>[2x]MVKYPKQLFLESKNSKMNSIEMKYGQDPAINRAEFHVYGGVRQSKRKSEAWEAAKRITKERGIPNYNPDLHLKGAQMGQKVLQTYRITGLDREWAGGEDTPAHKGWKPGTDIAGLEMDDLNYENNPAMQQCYDDMRRTAINGLSIAHETIERRFGKEVTPETINLYFEMLNHNIGAGAIMMEHTAETNPELV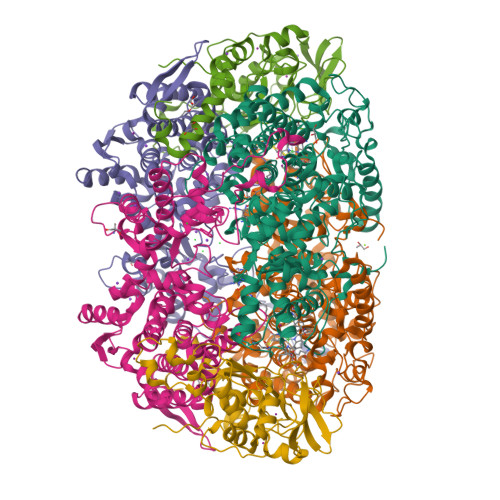KDSYAKCFTGNDELADALDQRFLIDINKMFPKYQADQIKAEVGDRIFQVARIPTMAVRTSDGGLSRAWVGQQASLAFLCAYDIPAGDAVTSDFVFTIKHGDVVFMGTQLPYRRAQRNNSAGGIALGYYSDCNQTSRTPEALEGLDGGIDPVKVIVEALTPGCVITDQGWLHNYLAGGSSGWSNYIISVYTDEVLEDYGYHGAIYAMDKWKCGVGEVPNTYENMMTIAEEVSRWSQKNYDEYPGLMEAHFGGSQRYSIQAAASGAAVGAMTGDPDLGNAAWHYNTPLCKEHYLRLGFYGHDLQDQQNMGHTYSYRSDQGIPYELKGPNYPDFAMNVGHMGGYIGIIAGAAHARGAAYSTNPIIKAAFADPNLQFDFRYPRREFGIGGLRQFMPAGERDAVIPPH;>MAYLTEKIDLYGDNGKVLESDIPLEAVTPVQNPAVRELASIFKRSVAVNLGGAQKALSTGHYANEYIHFPDIPNKDKLGIKSSPGGKYPPKSVKVRTMDLPLVDDADDIAARLKERLQVNPDDGTEVRVMKKGNVLYVKISEQLANTGVEYTTALTTTAQAMTDLVMEKYDLDFHASPLVHCAFYGRYPQTYEFMGGNVISLLAASCANEGPGFAMRNIMANHIVAATRKRTLEAVALSSTLEAIGHVEMGDAIGRWRRWQALVHACQGLNANNVVYDLVKEAGHGCTGDVVAATVGRALEDGIISVKKTLPSGYKFYTANDPSMWNAYVCAGLVAAVIVNQGAARAAQGVSSTLLYFNDLIEHETGLPHAGYGDGMGNGVSFSFFSHAIYGGGSPGIFSGNHIVTRHSKGFAIPVIAAAVSLDSGTAVYGPEATSGLVGDIFGEVDLIRRPMEAIASAAAEIKDKF[2x];>[2x]MVYQRQFLPADDRVTKNRKKVVDPSVKLEKIRTLSDKDFLTLIGHRHLGEAYRSVNPPLAEIGEPEDPIRELVPPTEGAKAGDRVCTIIMTDSVYNPPIAHYTRAWMYHNRFRGIDNGVYSGRVTLEMRERDLEEACRTLFETEICDASRDQVRQYTCTGHSCRLDPDGMMFDPIERCIMSGGNVVYQKDSFGNPVDTPINMGKPLSEEELIERTVVYRTDRGEPMTREGDPGAPDEEVREALQWSRRIQWLRMLGNMVPDKIKGM OXALYL-COENZYME A | 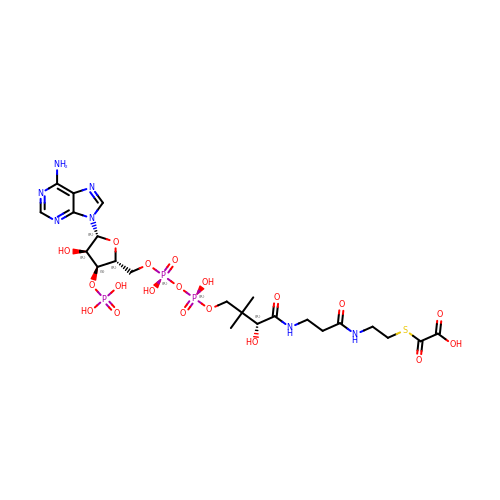C23 H36 N7 O19 P3 S | QVXMZFTWJVBUHP-IBOSZNHHSA-N>ENLTPQHMASMALTGTDRVKRGMAEMQKGGVIMDVVNAEQAKIAEAAGAVAVMALERVPADIRAAGGVARMADPTVIEEVMNAVSIPVMAXVRIGHYVEARVLEALGVDYIDESEVLTPADEEFHIDKRQFTVPFVCGCRDLGEAARRIAEGASMLRTKGEPGTGNIVEAVRHMRKVNAQIRKVVNMSEDELVAEAKQLGAPVEVLREIKRLGRLPVVNFAAGGVTTPADAALMMHLGADGVFVGSGIFKSENPEKYARAIVEATTHYEDYELIAHLSKGLGGAMRGIDIATLLPEHRMQERGWA[8x];>ENLTPQHMASMALTGTDRVKRGMAEMQKGGVIMDVVNAEQAKIAEAAGAVAVMALERVPADIRAAGGVARMADPTVIEEVMNAVSIPVMAKVRIGHYVEARVLEALGVDYIDESEVLTPADEEFHIDKRQFTVPFVCGCRDLGEAARRIAEGASMLRTKGEPGTGNIVEAVRHMRKVNAQIRKVVNMSEDELVAEAKQLGAPVEVLREIKRLGRLPVVNFAAGGVTTPADAALMMHLGADGVFVGSGIFKSENPEKYARAIVEATTHYEDYELIAHLSKGLGGAMRGIDIATLLPEHRMQERGWA[3x];> ENLTPQHMASMALTG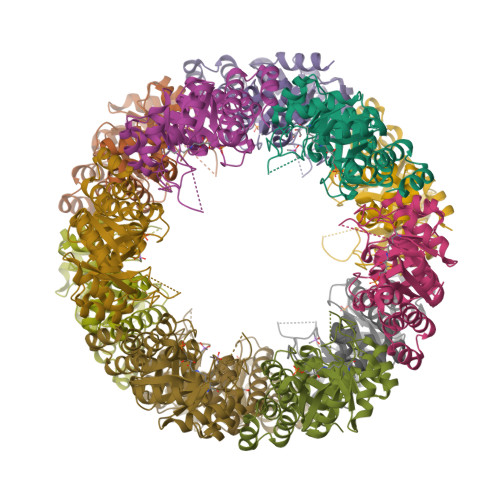TDRVKRGMAEMQKGGVIMDVVNAEQAKIAEAAGAVAVMALERVPADIRAAGGVARMADPTVIEEVMNAVSIPVMAXVRIGHYVEARVLEALGVDYIDESEVLTPADEEFHIDKRQFTVPFVCGCRDLGEAARRIAEGASMLRTKGEPGTGNIVEAVRHMRKVNAQIRKVVNMSEDELVAEAKQLGAPVEVLREIKRLGRLPVVNFAAGGVTTPADAALMMHLGADGVFVGSGIFKSENPEKYARAIVEATTHYEDYELIAHLSKGLGGAMRGIDIATLLPEHRMQERGW4-[(3-chloropyridin-2-yl)sulfamoyl]benzene-1-sulfonic acid 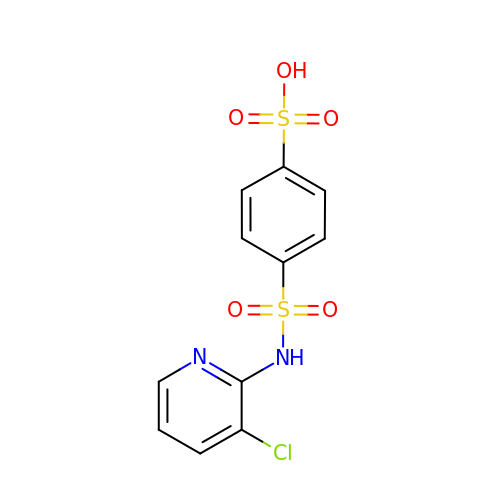| C11 H9 Cl N2 O5 S2 | HCEVZVCXFTUKMF-UHFFFAOYSA-N>MSFFHASQRDALNQSLAEVQGQINVS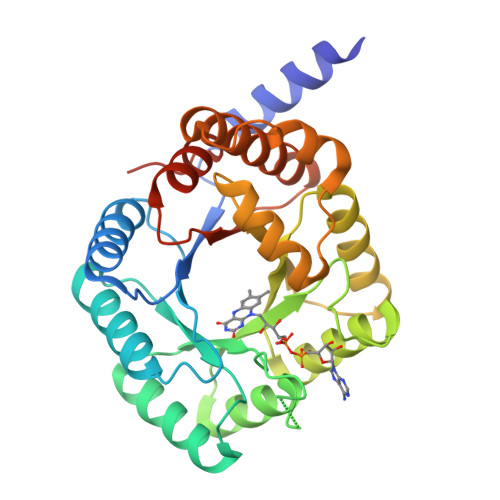FEFFPPRTSEMEQTLWNSIDRLSSLKPKFVSVTYGANSGERDRTHSIIKGIKDRTGLEAAPHLTCIDATPDELRTIARDYWNNGIRHIVALRGALPPGSGKPEMYASDLVTLLKEVADFDISVAAYPEVHPEAKSAQADLLNLKRKVDAGANRAITQFFFDVESYLRFRDRCVSAGIDVEIIPGILPVSNFKQAKKFADMTNVRIPAWMAQMFDGLDDDAETRKLVGANIAMDMVKILSREGVKDFHFYTLNRAEMSYAICHTLGVRPGLLEHHHHHH[3x]> PTPSAPV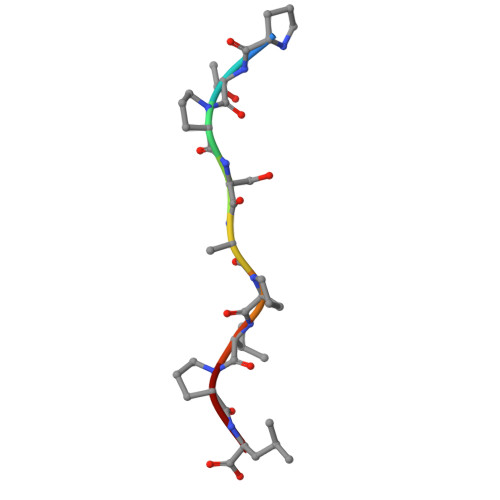PL> QGGAAAPISSHARLDKSNFQQPYITNRTFMLAKEASLADNNTDVRLIGEKLFHGVSMSERCYLMKQVLNFTLEEVLFPQSDRFQPYMQEVVPFLARLSNRLSTCHIEGDDLHIQRNVQKLKDTVKKLGESGEIKAIGE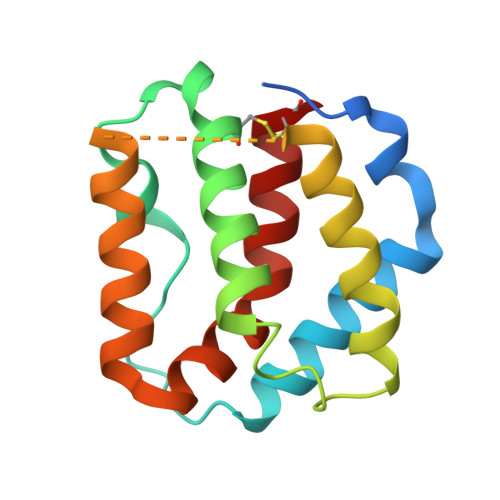LDLLFMSLRNACI>[2x]MSVLISGASGYIAKHIVRVLLEQNYKVIGTVRSQDKADKLLKQYNNPNLSYEIVPEIANLDAFDDIFKKHGKEIKYVIHAASPVNFGAKDLEKDLVIPAINGTKNMFEAIKKYAPDTVERVVMTASYASIMTPHRNNDPTLTLDEETW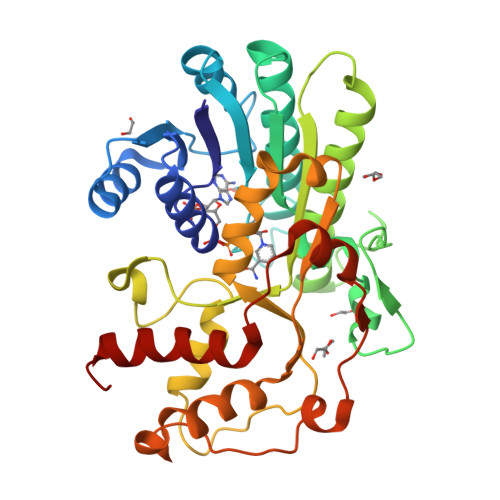NPVTEENAYENVVTAYCASKTFAEKEAWKFVKENSDAVKFKLTTIHPGFVFGPQNFDEDVTKKLNGTCEIINGLLHAPFDTKVEKTHFCQFIDVRDVAKTHVLGFQKDELINQRLLLCNGAFSQQDIVNVFNEDFPELKGQFPPEDKDTDLNKGVTGCKIDNEKTKKLLAFEFTPFHKTIHDTVYQILHKEGRV2,4-bis(chloranyl)-N-[3-cyano-6-[(4-hydroxyphenyl)methyl]-5,7-dihydro-4H-thieno[2,3-c]pyridin-2-yl]-5-morpholin-4-ylsulfonyl-benzamide 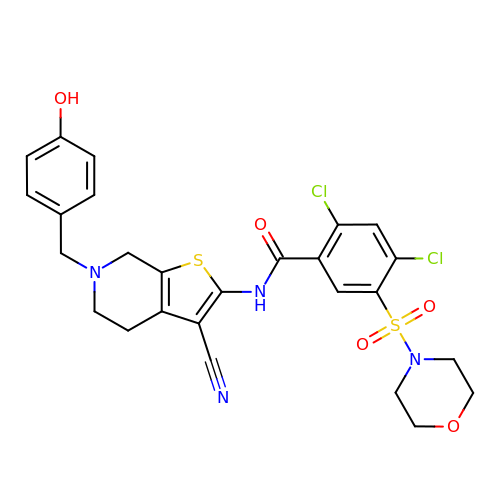| C26 H24 Cl2 N4 O5 S2 | VSLIZFRORGVSOU-UHFFFAOYSA-N> AQITGRPEWIWLA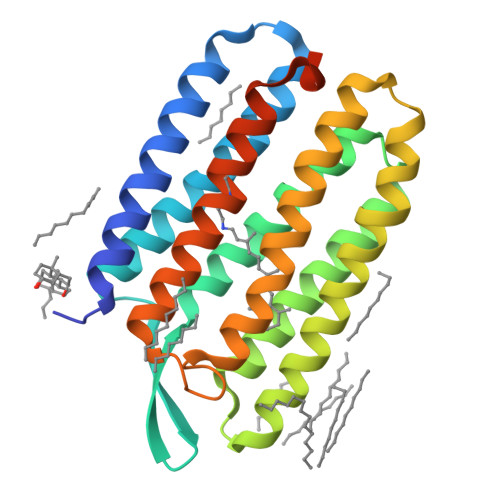LGTALMGLGTLYFLVKGMGVSDPDAKKFYAITTLVPAIAFTMYLSMLLGYGLTMVPFGGEQNPIYWARYADWLFTTPLLLLDLALLVDADQGTILALVGADGIMIGTGLVGALTKVYSYRFVWWAISTAAMLYILYVLFFGFTSKAESMRPEVASTFKVLRNVTVVLWSAYPVVWLIGSEGAGIVPLNIETLLFMVLDVSAKVGFGLILLRSRAIFGEAEAPEPSAGDGAAATS3-{[(2R,5S)-5-{[(2S)-2-(AMINOMETHYL)PYRROLIDIN-1-YL]CARBONYL}PYRROLIDIN-2-YL]METHOXY}-4-CHLOROBENZOIC ACID 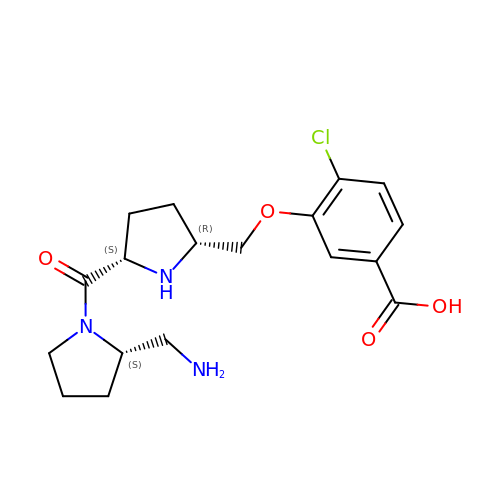| C18 H24 Cl N3 O4 | DUMYZIXJYDQLTO-IPYPFGDCSA-N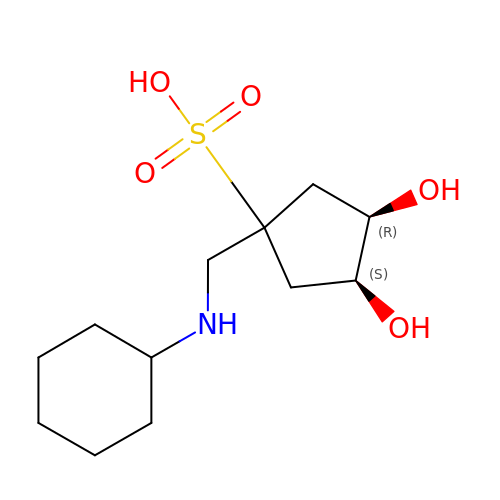(1s,3R,4S)-1-[(cyclohexylamino)methyl]-3,4-dihydroxycyclopentanesulfonic acid | C12 H23 N O5 S | RMLVAYWMDDDXFB-ZSBIGDGJSA-N>[7x]MSIPVTEFRQFSEQQPAFRVLKPWWDVFTDYLSVAMLMIGVFGCTLQVMQDKIICLPKRVQPAQNHSSLSNVSQAVASTTPLPPPKPSPANPITVEMKGLKTDLDLQQYSFINQMCYERALHWYAKYFPYLVLIHTLVFMLCSNFWFKFPGSSSKIEHFISILGKCFDSPWTTRALSEVSGEDSEEKDNRKNNMNRSNTIQSGPEGSLVNSQSLKSIPEKFVVDKSTAGALDKKEGEQAKALFEKVKKFRLHVEEGDILYAMYVRQTVLKVIKFLIIIAYNSALVSKVQFTVDCNVDIQDMTGYKNFSCNHTMAHLFSKLSFCYLCFVSIYGLTCLYTLYWLFYRSLREYSFEYVRQETGIDDIPDVKNDFAFMLHMIDQYDPLYSKRFAVFLSEVSENKLKQLNLNNEWTPDKLRQKLQTNAHNRLELPLIMLSGLPDTVFEITELQSLKLEIIKNVMIPATIAQLDNLQELSLHQCSVKIHSAALSFLKENLKVLSVKFDDMRELPPWMYGLRNLEELYLVGSLSHDISRNVTLESLRDLKSLKILSIKSNVSKIPQAVVDVSSHLQKMCIHNDGTKLVMLNNLKKMTNLTELELVHCDLERIPHAVFSLLSLQELDLKENNLKSIEEIVSFQHLRKLTVLKLWHNSITYIPEHIKKLTSLERLSFSHNKIEVLPSHLFLCNKIRYLDLSYNDIRFIPPEIGVLQSLQYFSITCNKVESLPDELYFCKKLKTLKIGKNSLSVLSPKIGNLLFLSYLDVKGNHFEILPPELGDCRALKRARLVVEDALFETLPSDVREQMKADALEVLFQ

Volume-regulated anion channels (VRACs) constitute a diverse family of ion channels that are ubiquitously expressed in mammalian cells. They are believed to be essential for maintaining cellular volume, as they are known to open in response to hypotonic stress, enabling efflux of anions and osmolytes, thereby preventing excessive cell swelling and burst. VRACs are hexamers composed of five closely related paralogues of the leucine-rich repeat-containing protein 8 family (termed LRRC8A to E). In contrast, when expressed on its own, the LRRC8C subunit forms a larger, heptameric assembly with weaker mutual subunit interactions and a different preferential arrangement of the LRRDs.

Previous studies of the structure of homomeric LRRC8C revealed its assembly as heptamer, which is larger than the hexameric organization of other characterized LRRC8 subunits and their heteromeric assemblies. Differences to WT become evident upon comparison of maps of LRRC8CV390L to wild-type LRRC8C homomers processed without application of symmetry (Fig. EV1). In the case of LRRC8CWT, the entire PDs are well-resolved for six subunits whereas density below the TMD towards the intracellular side is absent in one case (Figs. 3E and EV1A).>GSHMSKSDVFHLGLTKND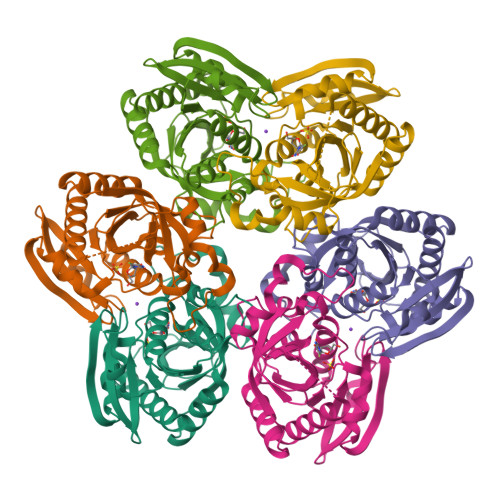LQGATLAIVPGDPDRVEKIAALMDKPVKLASHREFTTWRAELDGKPVIVCSTGIGGPSTSIAVEELAQLGIRTFLRIGTTGAIQPHINVGDVLVTTASVRLDGASLHFAPLEFPAVADFECTTALVEAAKSIGATTHVGVTASSDTFYPGQERYDTYSGRVVRHFKGSMEEWQAMGVMNYEMESATLLTMCASQGLRAGMVAGVIVNRTQQEIPNAETMKQTESHAVKIVVEAARRLL[2x]>MKYLLPTAAAGLLLLAAQPAMAMGWSHPQFEK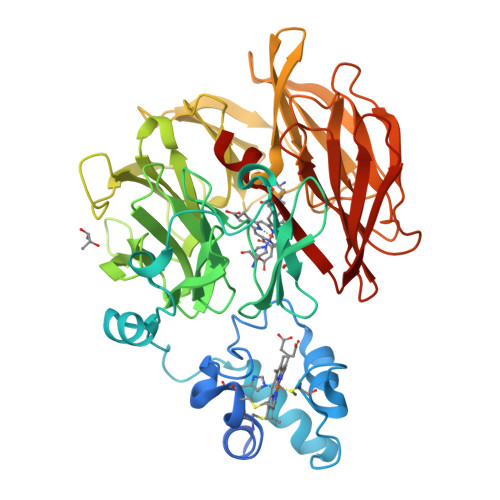ASGEAPGEALYRQHCQACHGAGRLGGSGPTLLPESLSRLKPAQAREVILHGRPATQMAGFAGQLDDAAADALVAYLYQAPPREPQWSAEDIRASQVQPHPLATLPSRPRFEADPLNLFVVVESGDHHVTILDGDRFEPIARFPSRYALHGGPKFSPDGRLVYFASRDGWVTLYDLYNLKVVAEVRAGLNTRNLAVSDDGRWVLVGNYLPGNLVLLDARDLSLVQVIPAADAQGQASRVSAVYTAPPRHSFVVALKDVHELWELPYANGKPVAPKRLAVADYLDDFSFSPDYRYLLGSSRQARGGEVIELDSGARVASIPLSGMPHLGSGIYWKRDGRWVFATPNISRGVISVIDLQNWKPLKEIVTDGPGFFMRSHADSPYAWTDTFLGKKHDEILLIDKQTLEIAHRLRPSPGKVAGHVEFTRDGRYALLSVWDRDGALVVYDAHSLEEVKRLPMNKPSGKYNVGNKIGYAEGTSH[2x]> GNPFEGVQLWANNYYRSEVHTLAIPQITDPALRAAASAVAEVPSFMWLDTLDKTPLMEQTLADIRTANKNGGNYAGQFVVYDLPDRDCAALASNGEYSIADGGVAKYKNYIDTIRQIVVEYSDIRTLLVIEPDSLANLVTNLGTPKCANAQSAYLECINYAVTQLNLPNVAMYLDAGHAGWLGWPANQDPAAQLFANVYKNASSPRALRGLATNVANYNAWSIASPPSYTSPNPNYDEKHYIEAFAPLLRNQGFDAKF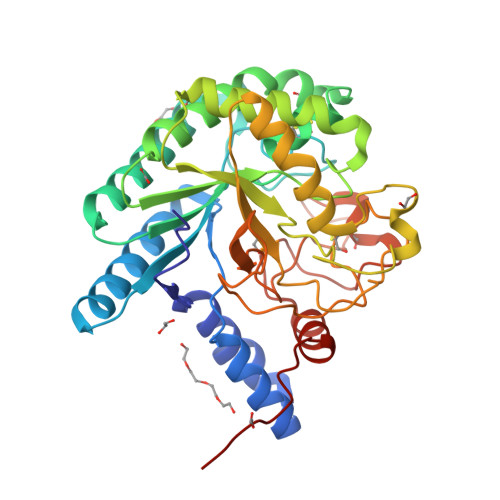IVDTGRNGKQPTGQLEWGHWCNVKGTGFGVRPTANTGHELVDAFVWVKPGGESDGTSDSSAPRFDSHCALPDALQPAPQAGAWFQAYFVQLLTNANPSFLHHHHHH>SNAMDQQFVAQLEQALGAIVQPTGSLKDATKTLQSQFYTQSAALPALIHILQNSSNDGIKQLAGVEARKQVSKHWGSLDAATQTSVKQSLLNSAFNEGKDAVRHANARVIASIGSEELDEKKWPELIPNLLQAACDSNPKIRETAIFIILSLLESFNANLALHIDDFLNLFAQTINDSASLETRSLSAQALSYVSSLIEEEGEINPQYAAKFASLIPSVVQVLDATIREGDTTNTKLIFNCLNDFLLLDSQLTGNTIADLVKLALQIAVNSDVDEDIRVFAVQFVTSALVYRKSKINQAKLGPEITLAALKVASEEIDVEDELTNEDEAGENEENTPALTALRLISNASGELSPSQVGVPIIEHLPTMLSSSNPFERRSILLAISVLVTGSPDYTLSQFDKIIPATVTGLKDSEAVVQLAALKCIVQLSTNLQDEVARYHEQYLPLVIDIIDSAKHVVIYKYATLALDGLLEFIAHNDIIKYLDPLMNKLFQMLETQQSPKLRAAIVSAIGSCAFAAGSGFVPYFKTSVQYLQQFIQNVSQIEGLSEDDIELKALTFENISTMGRAVKSAAFAEYAEPLVNAAYEAIKTDSARLRESGYAFIANMAKVYGKDFAPFLQTIIPEIFKTLEQEEYQFNFDGDEDFLEGIEDLDEEELQSKFTVNTGIAYEKEVAAAALSELAIASKEHFLEYVEPSLKVLAEQVNESYGLKETALHSMWAIVKAVLLTANLKEGEYPKGVPSGSYVDASALAVIQTVREVSLNNVIEEVETSMVISVFQDLSEMLRLFGPIIIMDNGDSTHLDQLCREALSVLKGEHACQTIHFEEDVPEDEDLDASETEATLLDVALDIYVALSTNLVGGFAQVFTTAKPVILQLCQSKSKNKRSFAVGALSEIALGMRDENPFIQELLEALIISLTNDKSLEVRCNASYGVGLLIEYSSFDVSAIYSPVLKSLYEILSVADEKNLATEDDEATKEIVDRTFSNVCGCVARMILKHQNLVPLEHTIPALLSHLPF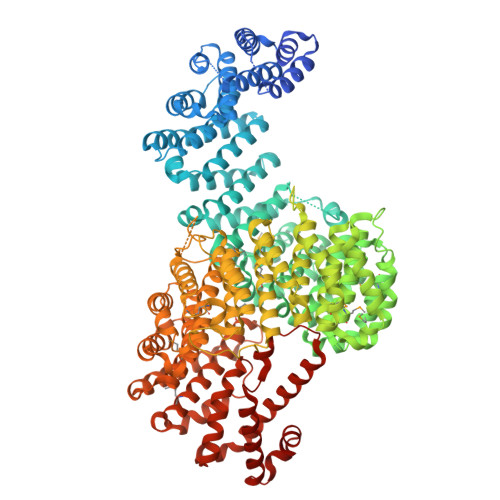NTAFEEYDPIFKLFLKLFQEQNSTIINEAPKVIAIFATVFEKESERIELETNSTLGREENLEKRKQFQSEEIKQQVIELLKHLNQQFNGAVAQNPVLAQVIA[2x]(2R)-2-[5-[(3aS,4S,6aR)-2-oxidanylidene-1,3,3a,4,6,6a-hexahydrothieno[3,4-d]imidazol-4-yl]pentanoylamino]-3-[[(5Z,10Z,14Z,19Z)-15-[[[(2R)-2-[5-[(3aS,4S,6aR)-2-oxidanylidene-1,3,3a,4,6,6a-hexahydrothieno[3,4-d]imidazol-4-yl]pentanoylamino]-3-sulfo-propanoyl]amino]methyl]-1,4,21,23-tetrahydroporphyrin-5-yl]methylamino]-3-oxidanylidene-propane-1-sulfonic acid | C48 H60 N12 O12 S4 | 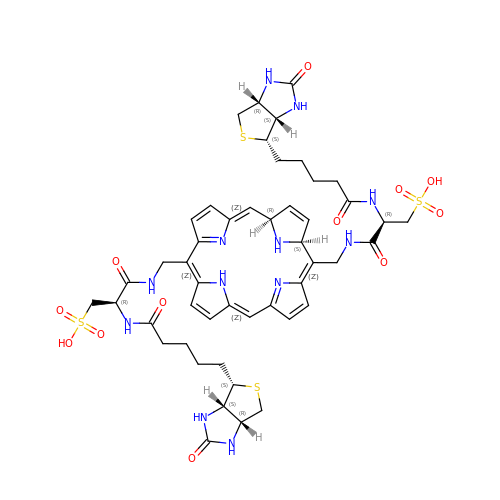GOHRVMOEJJKEAR-NBUULTOJSA-N> GSEGHRTLASTPALWASIPCPRSELRLDLVLPSGQSFRWREQSPAHWSGVLADQVWTLTQTEEQLHCTVYRGDKS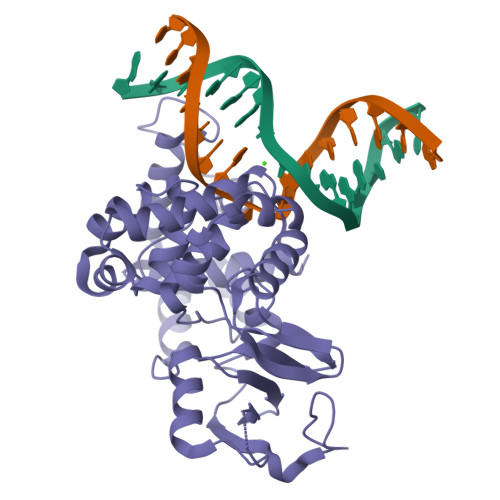QASRPTPDELEAVRKYFQLDVTLAQLYHHWGSVDSHFQEVAQKFQGVRLLRQDPIECLFSFICSSNNNIARITGMVERLCQAFGPRLIQLDDVTYHGFPSLQALAGPEVEAHLRKLGLGYRARYVSASARAILEEQGGLAWLQQLRESSYEEAHKALCILPGVGTKVADCICLMALDKPQAVPVQVHMWHIAQRDYSWHPTTSQAKGPSPQTNKELGNFFRSLWGPYAGWAQAVLFSADLRQ>[2x]MGSITENTSWNKEFSAEAVNGVFVLCKSSSKSCATNDLARASKEYLPASTFKIPNAIIGLETGVIKNEHQVFKWDGKPRAMKQWERDLTLRGAIQVSAVPVFQQIAREVGEVRMQKYLKKFSYGNQNISGGIDKFWLEGQLRISAVNQVEFLESLYLNKLSASKENQLIVKEALVTEAAPEYLVHSKTGFSGVGTESNPGVAWWVGWVEKETEVYFFAFNMDIDNESKLPLRKSIPTKIMESEGIIG

pmcβ-Lactamases are a major mechanism of resistance to the clinically vital β-lactam antibiotics, with >2,000 different β-lactamases reported (1). β-Lactamases are grouped into classes A, C, and D, which employ a nucleophilic serine in catalysis (serine β-lactamases, SBLs), and class B, which employ metal ions in catalysis (2). Penam sulfones, which are structurally related to penicillins, inhibit clinically important serine β-lactamases (SBLs) by forming transiently stable covalent complexes, thereby protecting β-lactam antibiotics from hydrolysis. Oxidation of penams to their sulfone state promotes bifurcation of their reaction with SBLs at the acyl–enzyme stage to give transiently inactivating species that are more resistant to hydrolysis than the nascent AEC 2, turning penam sulfones into transient inactivators of SBLs. Studies on the mechanism of the new SBLi enmetazobactam employing mass spectrometry and X-ray crystallography inform on its mode of action and also lead to reevaluation of mechanisms of current clinically important SBLi.

To test for formation of Dha-containing species 9, the −18-Da protein product was subjected to reaction with a thiol, a reaction used in protein engineering to introduce covalent modifications. No reaction was observed on incubation of unmodified OXA-10 with β-mercaptoethanol (BME, 1,000 equiv.), as monitored by SPE-MS. By contrast, after complete modification of OXA-10 to give the −18-Da species (8 h with excess tazobactam; validated by SPE-MS) and subsequent addition of BME (1,000 equiv.), ∼80% of the −18-Da protein was converted to a +60-Da species (relative to unmodified OXA-10) within 2 h. This observation is in agreement with the addition of BME to Dha 9 to give 2-hydroxyethyl-cysteine (Dha-BME, 17). The extent of conversion to the +60-Da species 17 was increased to ≥98% by simultaneous incubation of OXA-10 with tazobactam (100 equiv.) and BME (1,000 equiv.) for 12 h and was decreased by prolonged incubation with tazobactam prior to BME addition. With OXA-10 treated simultaneously with tazobactam and BME, a +60-Da modification (in agreement with Dha-BME 17) was observed at Ser67. Samples of OXA-10, treated with tazobactam or tazobactam in combination with BME (with full conversion to the respective −18- and +60-Da species verified by SPE-MS) were crystallized. Notably, although generation of small amounts of the L(2R)-epimer cannot be ruled out, the addition of BME to Dha 9 appears stereoselective with only the D(2S)-residue being observed. In both chains the hydroxyethyl oxygen is oriented so that the OH is positioned in the same location as the deacylating water in the active site of unmodified OXA-10. The different stereoselectivities observed for intermolecular (BME) and intramolecular (Lys) additions to Dha 9 are of interest from the perspective of use of Dha in protein engineering.>GIDPFTFENATSDAINQDMMLYIERIAKIIQKLPKRVHINVRGFTDDTPLVKTRFKSHYELAANRAYRVMKVLIQYGVNPNQLSFSSYGSTNPIAPNDSLENRMKNN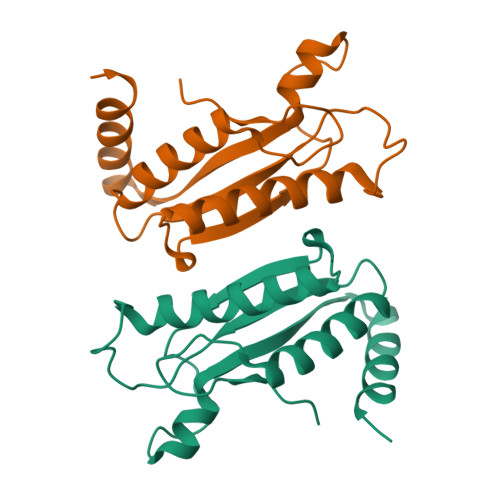RVEIFFSTDANDLSKIHSILDNEFNPHKQQE[16x]>[48x]MNNLYRDLAPVTEAAWAEIELEAARTFKRHIAGRRVVDVSDPGGPVTAAVSTGRLIDVKAPTNGVIAHLRASKPLVRLRVPFTLSRNEIDDVERGSKDSDWEPVKEAAKKLAFVEDRTIFEGYSAASIEGIRSASSNPALTLPEDPREIPDVISQALSELRLAGVDGPYSVLLSADVYTKVSETSDHGYPIREHLNRLVDGDIIWAPAIDGAFVLTTRGGDFDLQLGTDVAIGYASHDTDTVRLYLQETLTFLCYTAEASVALSH

Encapsulins are a class of BMCs characterised by their conserved subunit (Enc), which self-assembles to encapsulate enzymatically active cargoes and can remain porous to cargo substrates. The overall structure of Enc subunits across species with different T numbers is conserved and consists of a peripheral domain (P-domain), an axial domain (A-domain), and an extension loop (E-loop). T = 1 encapsulins of Mycobacterium tuberculosis, the causative agent of tuberculosis, and the closely related Mycobacterium marinum, are known to encapsulate the DyP as a core cargo with iron storage ferritin protein (BfrB)28 and FolB as possible secondary cargoes. In vitro cryo-electron microscopy (EM) single-particle analysis of the Mycobacterium tuberculosis encapsulin was used to obtain three structures of the encapsulin shell in intermediate states, as well as a 2.3 Å structure of the fully assembled shell.

In addition, we studied partial encapsulin structures to characterise stable encapsulin shell intermediates in vitro, by using low pH conditions to disassemble encapsulin shells, followed by reassembly at neutral pH. To explore the structural landscape of encapsulin shell formation, we used 2D and 3D (focused) classification and local symmetry to determine the structure of different stable encapsulin intermediates in an incomplete assembly state. This resulted in structures of three distinct intermediates of the encapsulin shell; a 48-mer (3,427 particles, 5.4 Å), a 52-mer (4,378 particles, 4.5 Å) and a 54-mer (6,294 particles, 4.6 Å). All three intermediates have an even number of monomers, appear to be closed on one side of the shell, and miss subunits on the other end. All three stable intermediates have an overall icosahedral structure with RMSD values for the 48,52 and 54-mer compared to the structure of the full shell of 1.08 Å, 0.60 Å and 2.66 Å respectively, although the 54-mer is, compared to the full encapsulin, flattened in one direction and elongated perpendicularly to it. The 48-mer and 52-mer retain their icosahedral geometry, whereas the 54-mer has a flattened appearance. The 48-mer has 39 fully resolved Enctb subunits (defined as cross-correlation value > 0.75) and 9 are less well resolved (defined as a cross-correlation value 0.5 to 0.75). The 48-mer and the 52-mer differ primarily by the addition of two more Enctb dimers along the edge, around a point of threefold symmetry. The addition of these dimers appears to increase the stability of Enctb subunits that previously were located directly on the edge of the hole. On the edges of the intermediate encapsulin shells, we observed many points of three and fivefold symmetry with one or more Enctb subunits missing. However, all dimers (in total 77) have both Enctb subunits present, and where a subunit around five or three fold symmetry is missing, its dimeric partner is also missing.>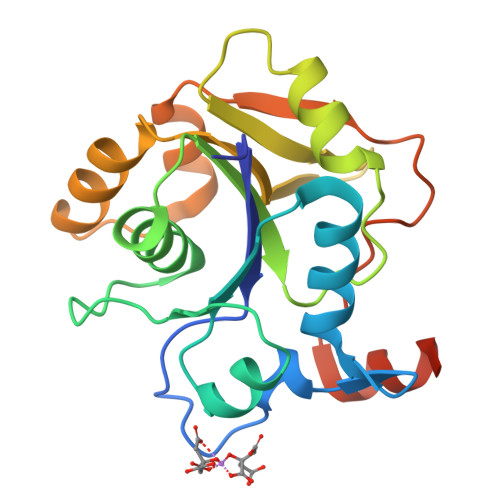 MNLMTTITGVVLAGGKARRMGLVDKGLLELNGKPLWQHVADALMTQLSHVVVNANRHQEIYQASGLKVIEDSLADYPGPLAGMLSVMQQEAGEWFLFCPCDTPYIPPDLAARLNHQRKDAPVVWVHDGERDHPTIALVNRAIEPLLLEYLQAGERRVMVFMRLAGGHAVDFSDHKDAFVNVNTPEELARWQEKRSHHHHHH> MGPSLDFALSLLRRNIRQVQTDQGHFTMLGIRDRLAVLPRHSQPGKTIWIEHKLVNVLDAVELVDEQGVDLELTLITLDTNEKFRDITKFIPENISTASDATLVINTEHMPSMFVPVGDVVQYGFL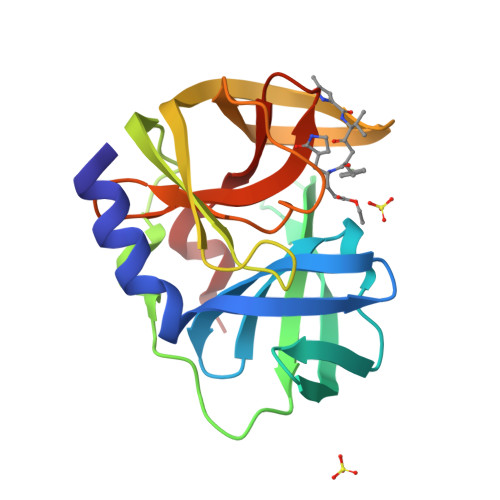NLSGKPTHRTMMYNFPTKAGQCGGVVTSVGKIIGIHIGGNGRQGFCAGLKRSYFAS>[6x]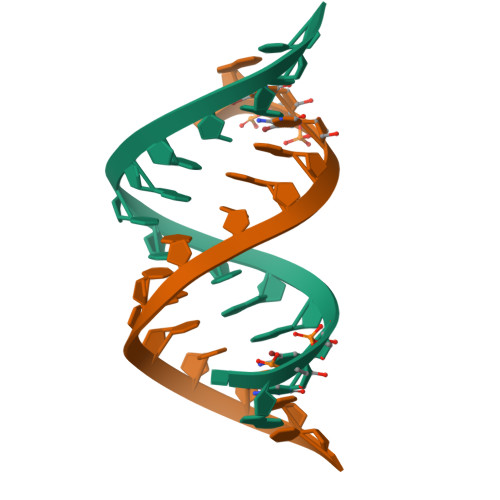UGCCAGUUCGCUGGC>[6x]MEFKKVAKETAITLQSYLTYQAVRLISQALSETNPGQAIWLGEFSKRHPIQESDLYLEAMMLENKELVLRILTVREN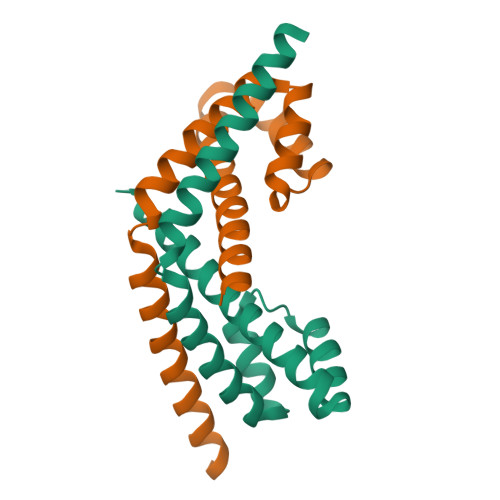LAEGVLEFLPEMVLSQIKQSNGNHRRSLLERLTQVDSSSTDQTEPNPGESDTSEDSE> MAVVIEPITNEDLTTKVVDGTGIFDELMTAANAHLSAQWDMERITGTQYAEVYLGQLTAVLQQAVTFLIEKD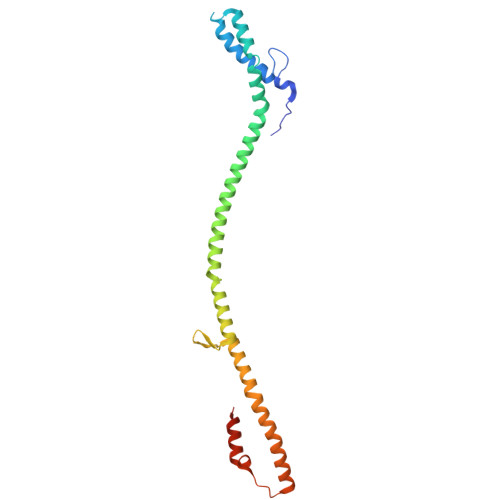KTYLNNLLINAQIELANKQIELADKELEKADKEIELLELNKELIAQKVKTEKAQISDTVDSVPVTGIIGAQIALYKQQKDGFIRDAEQKALKIISDTWITRKTVDDGTPLPTGFDTAAVDAFTRKVADGVSVNY>MKFDVIIIGGSYAGLSAALQLGRARKNILLVDAGERRNRFASHSHGFLGQDGKAPGEIIAEARRQIERYPTIHWVEGRVTDAKGSFGEFIVEIDGGRRETAGRLILAMGVTDELPEIAGLRERWGSAVFHCPYCHGYELDQGKIGVIAASPMAIHHALMLPDWGETTFFTNGIVEPDADQHALLAARGVRVETTRIREI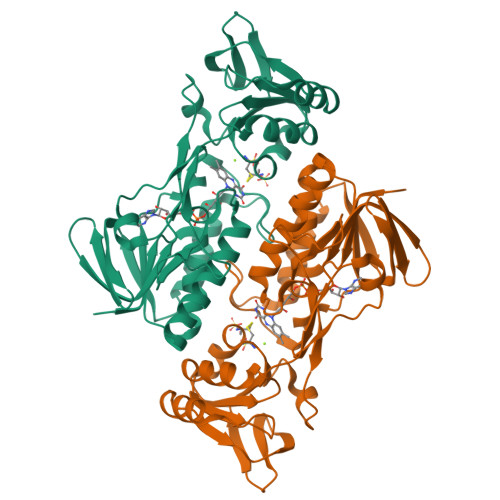AGHADVVLADGRSIALAGLFTQPKLRITVDWIEKLGCAVEEGPMGSTIVTDPMKQTTARGIFACGDVARPAGSVALAVGDGAMAGAAAHRSILFPEMR[2x]> GSSPSLEQDDGDEETSVVIVGKISFCPKDVLGHG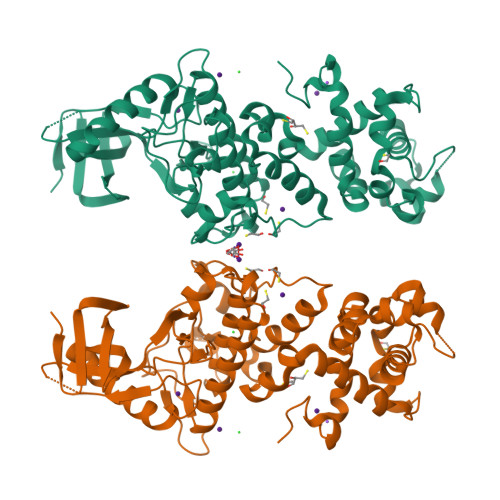AEGTIVYRGMFDNRDVAVKRILPECFSFADREVQLLRESDEHPNVIRYFCTEKDRQFQYIAIELCAATLQEYVEQKDFAHLGLEPITLLQQTTSGLAHLHSLNIVHRDLKPHNILISMPNAHGKIKAMISDFGLCKKLAVGRHSFSRRSGVPGTEGWIAPEMLSEDCKENPTYTVDIFSAGCVFYYVISEGSHPFGKSLQRQANILLGACSLDCLHPEKHEDVIARELIEKMIAMDPQKRPSAKHVLKHPFFWSLEKQLQFFQDVSDRIEKESLDGPIVKQLERGGRAVVKMDWRENITVPLQTDLRKFRTYKGGSVRDLLRAMRNKKHHYRELPAEVRETLGSLPDDFVCYFTSRFPHLLAHTYRAMELCSHERLFQPYYFHEPPEPQPPVTPDAL>MRPHRAFSPGLTGVLPLRETRHLVEVLRARVGDRFTVFDGEREALAEVVDLGPPLRYRVLEERRPEREVGVEVVLYVALLKGDKLAEVVRAATELGATRIQPLVTRHSVPKEMGEGKLRRLRAVALEAAKQSGRVVVPEVLPPIPLKAVPQVAQGLVAHVGATARVREVL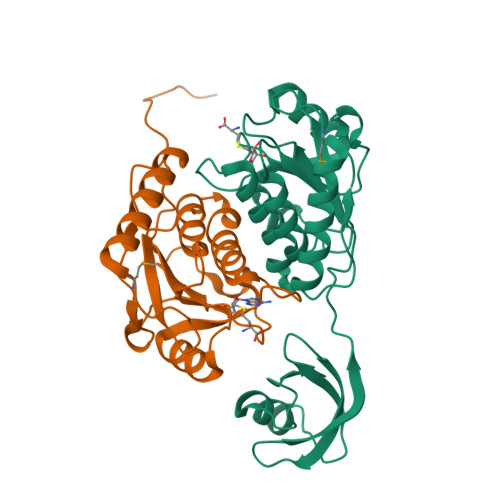DPEKPLALAVGPEGGFAEEEVALLEARGFTPVSLGRRILRAETAALALLALCTAGEGR[2x]> MRGSHHHHHHGSACKLLFVCLGNICRSPAAENIMNAQIDQAGLGAKIVCDSAGTSSYHVGDSPDRRMTESLKKRGYRVQGRARQFFPEDFAEFDLILAMDGDNYRNILAQDPAGQYHHKVKMICDYTEK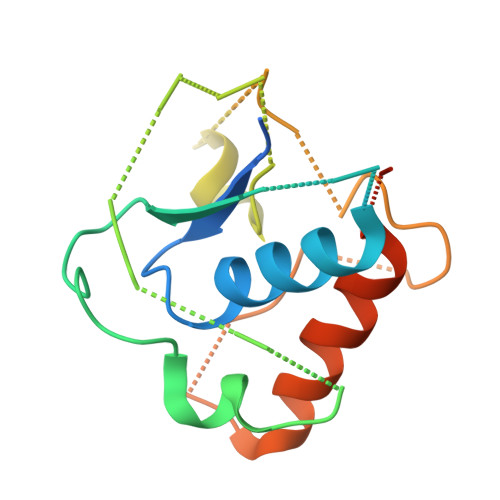FGDREVPDPYYGGQAGFEHVIDLLEDACGNLLTSLGKELVN>MDKFRMMFQFLQSNQESFMNGICGIMALASAQMYSSFEFSCPCMPEYNYTYGIGLLIIPPIWFFLLGFVLNNNVSVLAEEWKRPTGRRTKDPSVLRYMLCSITQRSLIAPAVWVSVTLMDGKSFLCAFSINLDIEKFGNASLVIGMTETEKLKFLA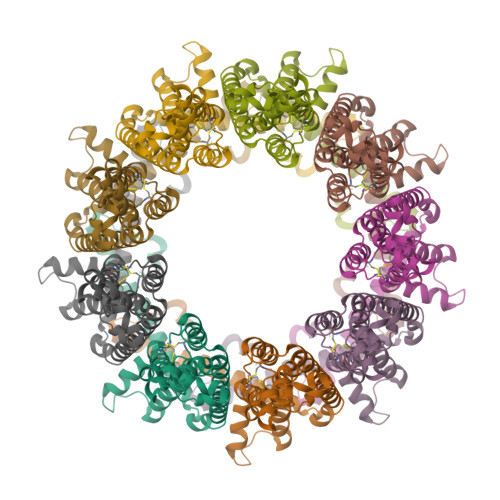RIPCKDLFEDNEVRVAATRYIKCISQACGWMFLLMMTFTAFLIRAIRPCFTQASYRQEAYWAQYRANEDQLFQRTAEVHSRVLAANNVRRFFGFVALNKDDEELIANFPVEGTQPRPQWNAITGVYLYRENQGLPLYSRLHKWAQGLAGNGAAPDNVEMALLPSENLYFQ[9x]>[4x]MKLLRRIAAPAIALGIAMSTIVTPST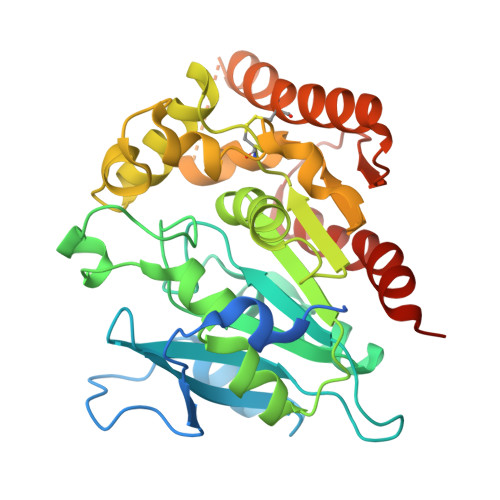AGAAEVTPADVAGDTALSTISDSAPADEASAPRWRAHVNAADERVKEMWAYSPSMDRNVPLVVITADESAGPRPVIYLLNGGDGGEGAANWVMQTDVLDFYLEKNVNVVIPMEGKFSYYTDWVEENASLGGKQMWETFLVKELPGPLEEKLNTDGQRAIAGMSMSATTSLLFPQHFPGFYDAAASFSGCAATSSLLPWEYLKLTLDRGNATPEQMWGPRGGEYNIYNDALINSDKLRGTELYVSNASGLAGEWESVDSPRFEGLNQQVQSIAMAETVVTGGIIEAATNKCTHDLKAKLDSAGIPADWNLRPTGTHSWGWWQDDLRGSWTTFARAFELEAHHHHHH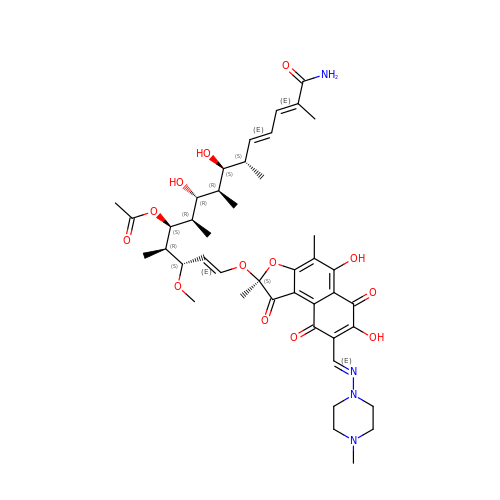(1E,3S,4R,5S,6R,7R,8R,9S,10S,11E,13E)-15-amino-1-{[(2S)-5,7-dihydroxy-2,4-dimethyl-8-{(E)-[(4-methylpiperazin-1-yl)imino]methyl}-1,6,9-trioxo-1,2,6,9-tetrahydronaphtho[2,1-b]furan-2-yl]oxy}-7,9-dihydroxy-3-methoxy-4,6,8,10,14-pentamethyl-15-oxopentadeca-1,11,13-trien-5-yl acetate | C43 H58 N4 O13 | ABIUUBSHMGGSQA-ONSLPDPNSA-N>[4x]MIKTEYNPKHSPIIEIEKEGELYKITIEVGKEVKHPNEPSHHIQWV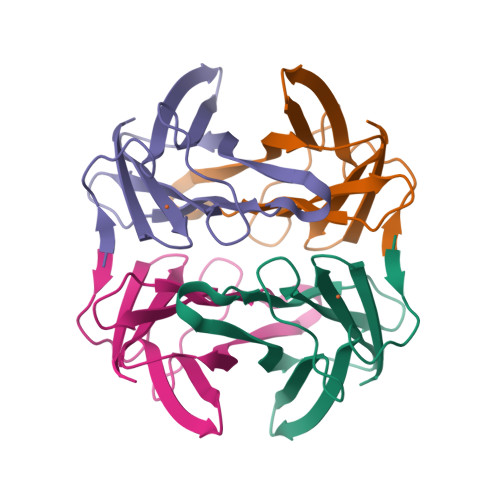DLYFEPEGKEPTHIARIEFKAHGEYNNYTEPKAIVYAKLEGKGKLIAISYCTLHGLWKTEKEL> GSHMN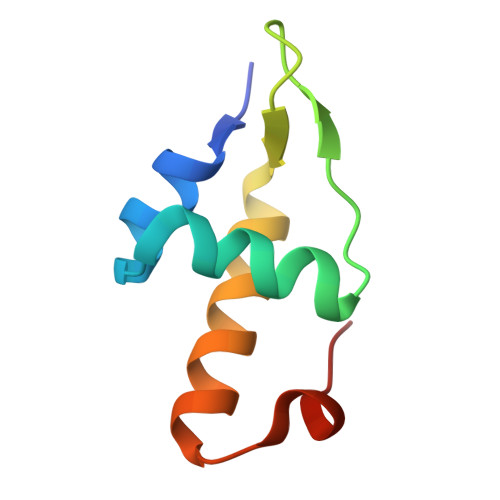TNMVASELGVSAKTVQRWVKQLNLPAERNELGHYSFTAEDVKVLKSVKKQISEGTAIQDIHLPK> SNAQEPILTITHQGQTVSATYQELLARSDLTIV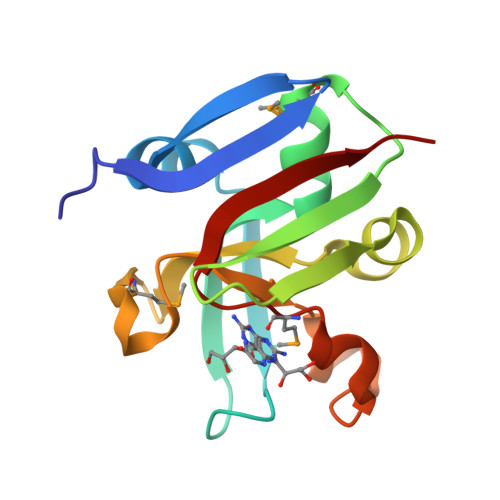TETPWTQGNTEFKGISAQALLAWMGVKQADLKVIALNKYWAEIPYSDIEKYNPVFAIQNNGKPMQIRDRGPIWSIYPLSSSGELDNEILHSRMVWQISSIEIITP> MAHHHHHHMLDHIGFNIADMKKSRAFYDAALSPLGIGHAMEFGDWVGYGRNGKPEFWIGAQKGAKLEGVLHVAFSAGTRSEVGRFYEAAIAAGGRD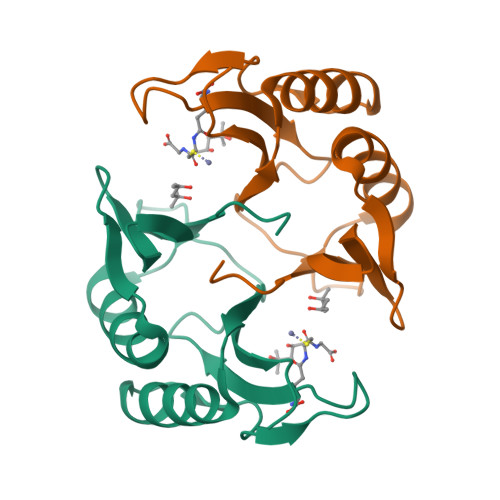NGKPGLRPHYHPDYYAAFVLDPDGHNIEVVCHLPE>EEEFQFLRCQQCQAEAKCPKLLPCLHTLCSGC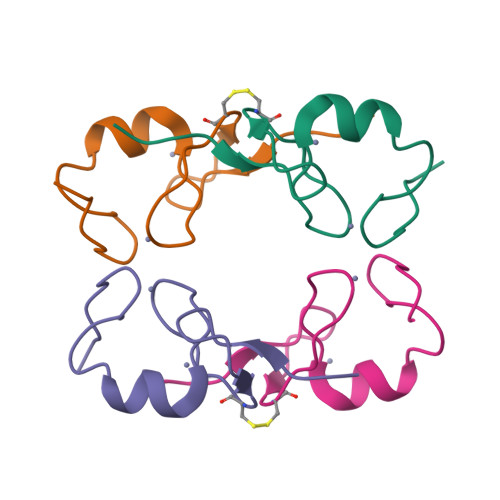LEASGMQCPICQAPWPLGA[4x]> MATEKKADVGKFVELPGAEMGKVIVRFPPEASGYLHIGHAKAALLNQHYQVNFKGKLIMRFDDTNPEKEKEDFEKVILEDVAMLHIKPDQFTYTSDHFETIMKYAEQLIQEGKAYVDDTPAEQMKAEREQRMESKHRNNCVNKNLQMWEEMKKGTEYGQTCCLRAKIDMNSNNGCMRDPTLYRCKNQPHPRTGTTYKVYPTYDFACPIVDSIEGVTHALRTTEYHDRDEQFYWIIEALGIRKPYIWEYSRLNLNNTVLSKRKLMWFVNEGLVDGWDDPRFPTVRGVLRRGMTVEGLKQFIAAQGSSRSVVNMEWDKIWSFNKKVIDPVAPRYTALLKDAVVPVNVPEAQEEMKEVAKHPKNADVGLKPVWYGSKVLIEGADAETLTEGEVVTFINWGNIIITKLNRNSSGKIVSIDTKLNLDNKDFKKTTKITWLAET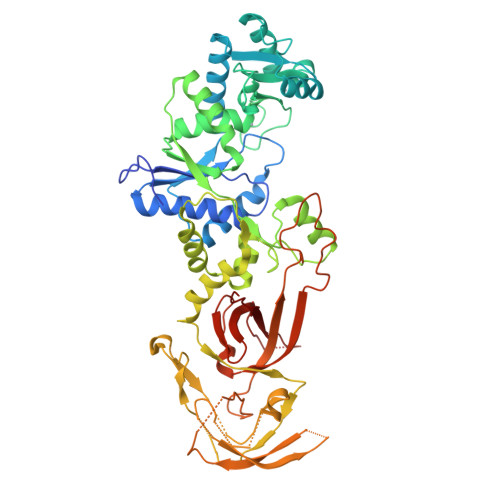PRAPLIPTVCVNYEHLITKPVLGKDEDFKQYINRNSKQEELMLGDPCLKDLKKGDIIQLQRRGFFICDQPYEPVSPYSCKEAPCILIYIPDGH>[2x]MGNIFSSMFDKLWGSNKELRILILGL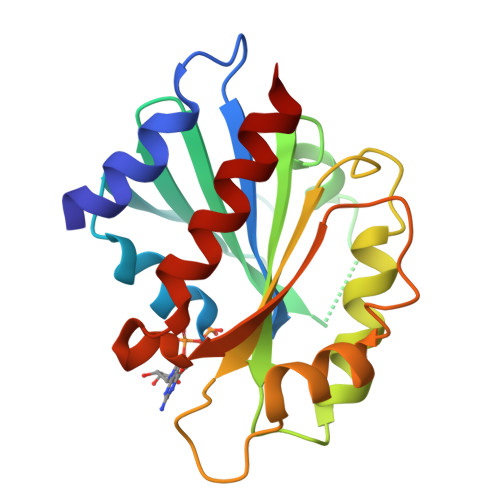DGAGKTTILYRLQIGEVVTTKPTIGFNVETLSYKNLKLNVWDLGGQTSIRPYWRCYYADTAAVIFVVDSTDKDRMSTASKELHLMLQEEELQDAALLVFANKQDQPGALSASEVSKELNLVELKDRSWSIVASSAIKGEGITEGLDWLIDVIKEEQL> MATDFSKLSKYVETLRVKPKQSIDLKKDFDTDYDHKMLTKEEGEELLNLGISKLSEIQEKLYASGTKSVLIVFQAMDAAGKDGTVKHIMTGLNPQGVKVTSFKVPSKIELSHDYLWRHYVALPATGEIGIFNRSHYENVLVTRVHPEYLLSEQ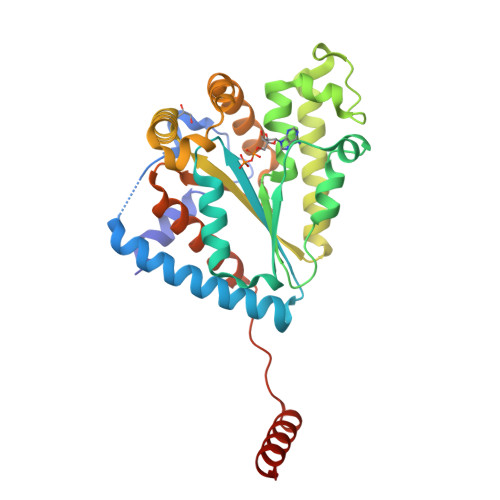TSGVTAIEQVNQKFWDKRFQQINNFEQHISENGTIVLKFFLHVSKKEQKKRFIERIELDTKNWKFSTGDLKERAHWKDYRNAYEDMLANTSTKQAPWFVIPADDKWFTRLLIAEIICTELEKLNLTFPTVSLEQKAELEKAKAELVAEKSSD>[2x]MGNKYRVRKNVLHLTDTEKRDFVRTVLILKEKGIYDRYIAWHGAAGKFHTPPGSDRNAAHMSSAFLPWHREYLLRFERDLQSINPEVTLPYWEWETDAQMQDPSQSQIWSADFMGGNGNPIKDFIVDTGPFAAGRWTTIDEQGNPSGGLKRNFGATKEAPTLPTRDDVLNALKITQYDTPPWDMTSQNSFRNQLEGFINGPQLHNRVHRWVGGQMGVFPTAPNDPVFFLHHANVDRI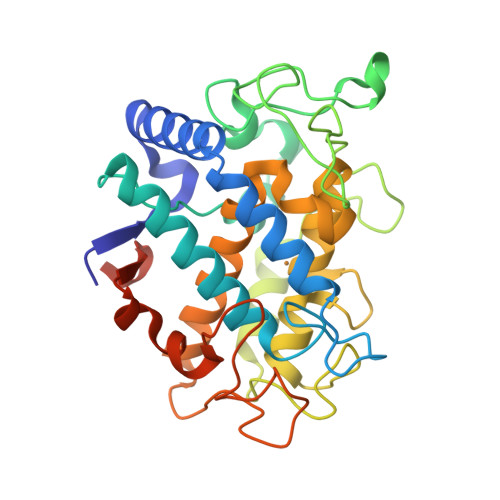WAVWQIIHRNQNYQPMKNGPFGQNFRDPMYPWNTTPEDVMNHRKLGYVYDIELRKSKRSSHHHHHH> MEQKRLERESLEKQPKITLEEFIETERGKLDKSKLTPITIANFAQWKKDHVIAKINAEKKLSSKRKPTGREIILKMSAENKSFETDNADMPDDVTQGSAWDLTEFTDALKKADHQDDGG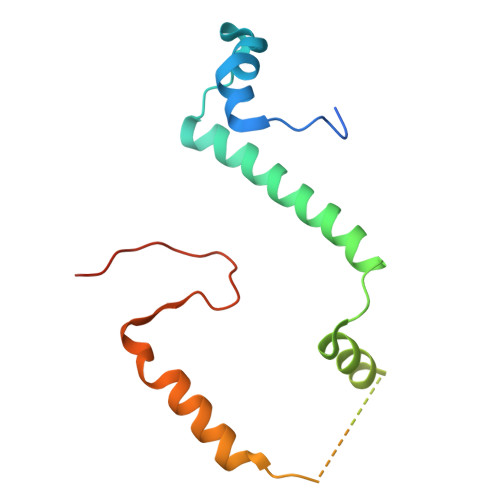IKDYGDGSNPTFDIKKANSATLA> MQNIPPQVQAMLGQLESYQQQLQLVVQQKQKVQLELTEAKKALDEIESLPDDAVVYKTVGTLIVKTTKDKAVAELKEKIETLEVRLNALERQEKKLNEKLKELTAQIQSALRPP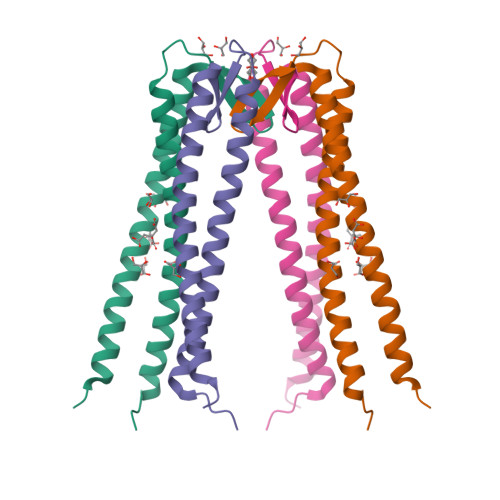TAG>[2x]GMSEQERIQECLRKEIRSLLI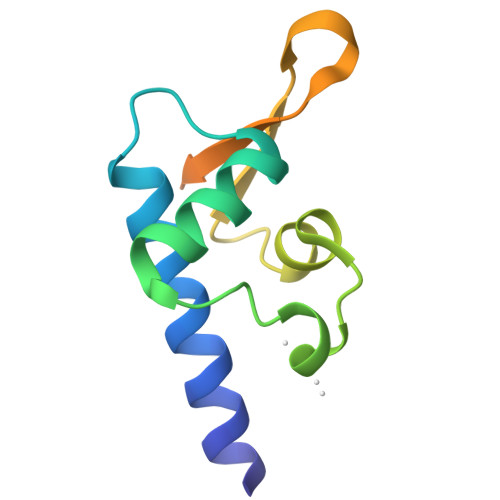STKDGLSPQELEKEYLLMVGNHLPLRILGYRSTMELVLDMPDVVRVCPGAGGTVILKAIPDESTKGIASLVAKQRSSHKLR>[2x]MNSELDYYEKFEEVHGILMYKDFVKYWDNVEAFQARPDDLVIATYPKSGTTWVSEIVYMIYKEGDVEKCKEDVIFNRIPFLECRKENLMNGVKQLDEMNSPRIVKTHLPPELLPASFWEKDCKIIYLCRNAKDVAVSFYYFFLMVAGHPNPGSFPEFVEKFMQGQVPYGSWYKHVKSWWEKGKSPRVLFLFYEDLKEDIRKEVIKLIHFLERKPSEELVDRIIHHTS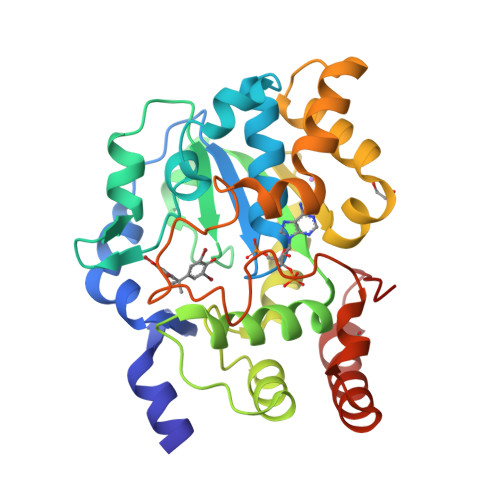FQEMKNNPSTNYTTLPDEIMNQKLSPFMRKGITGDWKNHFTEALNEKFDKHYEQQMKESTLKFRTEI> MESLPVIAAPSMWTRPQIKDFKEKIQQDADSVITVGRGEVVTVRVPTHEEGSYLFWEFATDNYDIGFGVYFEWTDSPNTAVSVHVSESSDDDEEEEENIGCEEKAKKNANKPLLDEIVPVYRRDCHEEVYAGSHQYPGRGVYLLKFDNSY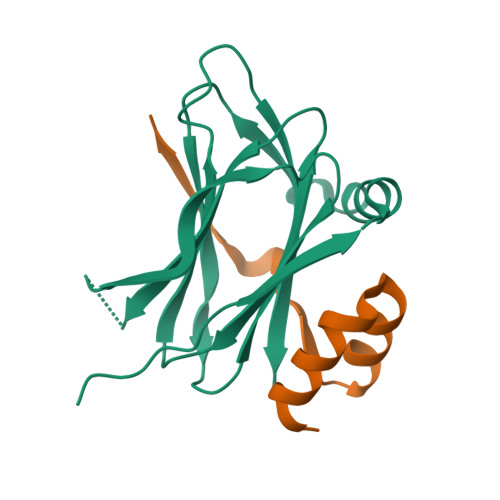SLWRSKSVYYRVYYTR;> GPLQYKDLKIDIKTSPPPECINDALQAVDSQEVRDYCEKKGWIVNITSQVQTERNINR> TVPVKLKPGMDGPKVKQWPLTEEKIKALVEICTEMEKEGKISKIGPENPYNTPVFAIKKKDSTKWRKLVDFRELNKRTQDFWEVQLGIPHPAGLKKKKSVTVLDVGDAYFSVPLDEDFRKYTAFTIPSINNKTPGIRYQY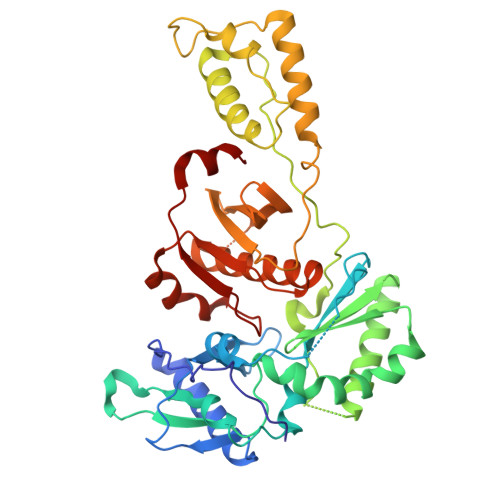NVLPQGWKGSPAIFQSSMTKILEPFRKQNPDIVIYQYMDDLYVGSDLEIGQHRTKIEELRQHLLRWGLTTPDKKHQKEPPFLWMGYELHPDKWTVQPIVLPEKDSWTVNDIQKLVGKLNWASQIYPGIKVRQLCKLLRGTKALTEVIPLTEEAELELAENREILKEPVHGVYYDPSKDLIAEIQKQGQGQWTYQIYQEPFKNLKTGKYARMRGAHTNDVKQLTEAVQKITTESIVIWGKTPKFKLPIQKETWETWWTEYWQATWIPEWEFVNTPPLVKLWYQ> MSGSHHHHHHSGSMSPSPIEEQATRLLKEVPLIDGHNDFPYMIRGWFRNDINGQ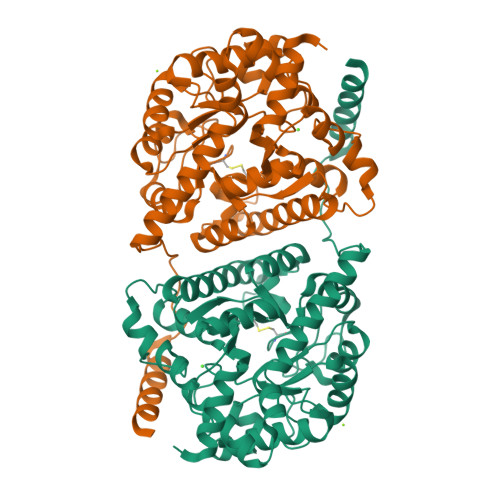DAHLYDMPIGQTDLQRLQKGLLGGQFWSAFVPCPKNPDKEVGSLEALRQTLQQLDVIHRLIERHPTILQFADSAASIWSSFRAGRVASLIGIEGLHQIADSVSALRMLHRLGVRYVTLTHNCHNAFADAATVSPELHGGLSRKGERLIRELNRMGMMIDLSHTSHEAQTQALRLSRAPVIYSHSSIYSLRAHARNVTDENLHLLHRNRGVVMICFLRELLASEADQATLAHVIDHIIYAGTRIGYEHVGIGSDFDGMLRGPDGLHDVSCYPALVAGLLERGVSEEDVKRVMGLNVIRVLEEVERVAAELQGAGEECLCDELDEVWNEDIKEQLTRERERVRKLGPQK>[2x]AGAGLDDPHKKEIAMELVSSAENSSLDWKAQYKYIEDIGDGRGY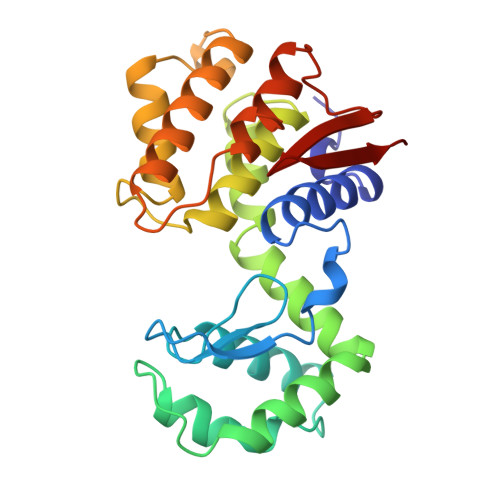TGGIIGFCSGTGDMLELVQHYTDLEPGNILAKYLPALKKVNGSASHSGLGTPFTKDWATAAKDTVFQQAQNDERDRVYFDPAVSQAKADGLRALGQFAYYDAIVMHGPGNDPTSFGGIRKTAMKKARTPAQGGDETTYLNGFLDARKAAMLTEAAHDDTSRVDTEQRVFLKAGNLDLNPPLKWKTYGDPYVINS>[2x]MAKDKEFQVLFVLT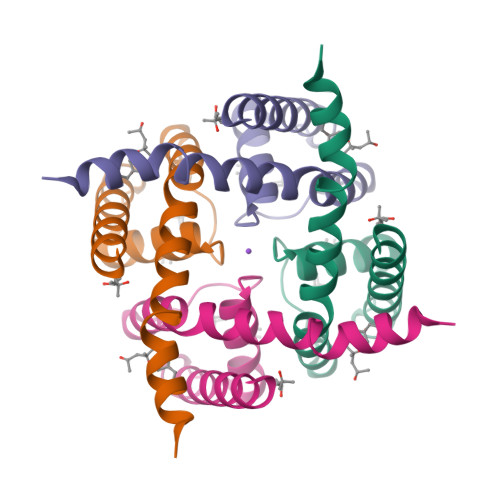ILTLISGTIFYSTVEGLRPIDALYFSVVTLTTVGNTPPPQTDFGKIFTILYIFIGIGLVFGFIHKLAVNVQLPSILSNLVPR>GAMADIGSEFMESTPTTIAFQVDCYLWHLKKMLSL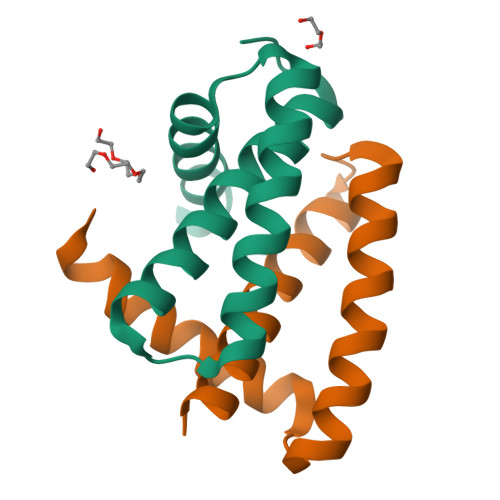MGEVDAPFEDRLRREQKALKGRSMTLGIDIQAATKAGYYKIKSITEDAM[2x]Annexin A2 is a non-EF-hand calcium-binding protein that is characterized by the ability to bind and aggregate (i.e. ‘annex’) anionic phospholipid membranes. AnxA2 preferentially binds to phospholipids and other anionic polymers and does not contain any canonical RNA- or DNA-binding motifs. Importantly, AnxA2 was shown to bind phosphorothioate oligonucleotides and has been implicated in the release of PS ASOs from endo-lysosomal compartments in productive ASO cellular trafficking. In the present study, we co-crystallized the C-terminal domain (CTD) core of AnxA2 with a PS 2′-MOE DNA gapmer ASO and found that unique hydrophobic interactions between PS groups and lysine and arginine residues account for the enhanced affinity of PS ASO to the protein surface.

From our crystallization trials, we obtained two types of AnxA2–ASO co-crystals that were used to solve two structures referred to as structure I and structure II, determined at 1.9 and 2.4 Å resolution, respectively. In structure II, it contains two copies of the complex (complex 1 and complex 2). The major difference between the two structures is that the nucleic acid is bound by AnxaA2 using two different interfaces. In structure II, only a small single-stranded part that comprised three or six (for complexes 2 and 1, respectively) of 15 nucleotides could be built in the model. In this crystal, the electron density indicated the presence of double-stranded nucleic acid that was formed by ASOs from complexes 1 and 2. Because of low quality of the electron density maps for nucleobases, it was not possible to establish the register of the ASO in structure II; therefore, an arbitrarily chosen dT sequence was built in the model. In structure II of the AnxA2–ASO complex, visible nucleotides were located in the vicinity of loop AB of domain II. Notably, this loop is the equivalent of loop IIIAB, which binds the PS group in structure I. The PS linkage makes van der Waals contacts with side chains of K115 and K119. In contrast to the distorted trajectory in structure I, the oligonucleotide backbone that is bound by the protein in structure II adopts a more canonical conformation.

>SDAERDALNIETAIKTKGVDEVTIVNILTNRSNAQRQDIAFAYQRRTKKELASALKSALSGHLETVILGLLKTPAQYDASELKASMKGLGTDEDSLIEIICSRTNQELQEINRVYKEMYKTDLEKDIISDTSGDFRKLMVALAKGRRAEDGSVIDYELIDQDARDLYDAGVKRKGTDVPKWISIMTERSVPHLQKVFDRYKSYSPYDMLESIRKEVKGDLENAFLNLVQCIQNKPLYFADRLYDSMKGKGTRDKVLIRIMASRSEVDMLKIRSEFKRKYGKSLYYYIQQDTKGDYQKALLYLCGGDD[2x]> MPLFFIRRPNFAWVVALFISLGGLLVIPFLPVAQYPNVAPPQITVTATYPGASAQVLTDSVTSVIEEELNGAKNLLYFESTSNANGIAEITVTFQPGTDPELAQVDVQNRLKKAEARMPQAVLTLGIQTEQATAGFLLIYSLRYKDGDKNANTTALADYAVRNVNNEIRRLPGVGKLQFFDSEAAMRVWIDPQKLVGYGLSIDDVNNAIRTQNVQVPAGAFGSTPGSSEQELTATLTVKGTLDNPEEFAAIVLRANQDGSRLTLGDVARIEVGSQDYNFGSRQDGKPAVAAAVQLSPGANAIQTAEAVKQRLTELSANFPDNVEFSVPYDTSRFVDVAIDKVIMTLIEAMVLVFLVMFLFLQNVRYTLIPSIVVPVCLLGTLTFMYLLGFSVNMMTMFGMVLAIGILVDDAIVVVENVERIMAEEGLAPVPATIKAMGQVSGAIIGITLVLSAVFLPLAFMAGSVGVIYQQFSLSLAVSILFSGFLALTFTPALCATLLKPIPVGHHEKTGFFGWFNRKFTSLTSRYTKLNDKLVPRAGRVMFIYLGVVVLMGFLYMRLPESFVPVEDQGYMIVDIQLPPGATRERTSAAGGELESFLMAREAVQTTFLVLGFSFSGMGENAAIAFPLLKDWSERDSSQSPEAESAAVNQHFANLDDGAIMAVPPPPVEGLGNSGGFALRLQDRAGLGRDALLAARDEVLGKVNGNPKFLYAMMEGLAEAPQLRLVIDREQARTLGVSFEAISSALSTAFGSSVINDFANAGRQ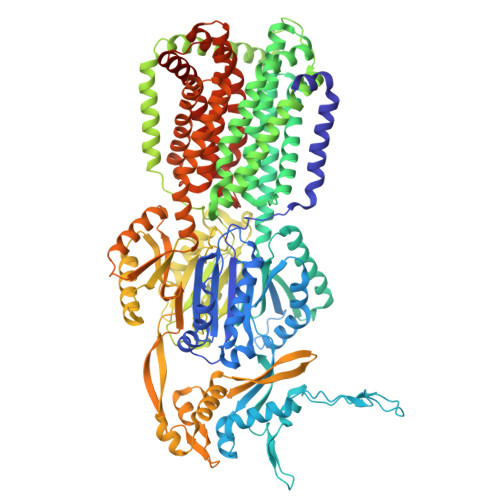QRVVVQAEQAERMTPESVLRLHVPNDSGSLVPLSAFVTTSWEEGPVQVARYNGYPSIRIAGDAAPGVSTGEAMLELERIAAELPEGIGYEWTGLSYQERVASGQATMLFALAITVVFLLLVALYESWAIPLTVMLIVPVGALGAVLAVTAIGLPNDVYFKVGLITVIGLAAKNAILIVEFAKDLWEDGYSLRDAAVEAARLRFRPIIMTSMAFMLGVVPLAIATGAGAASQRALGTGVLGGMLSATMLGVIFVPIFFVWVLSLLRTKPQQTDNHPLHKAE> GLPTMLTPGSNQFLTSDDFQSPSAMPQFDVTPEMKIPGEVHNLMEIAEVDSVVPVNNTKENINSMEAYR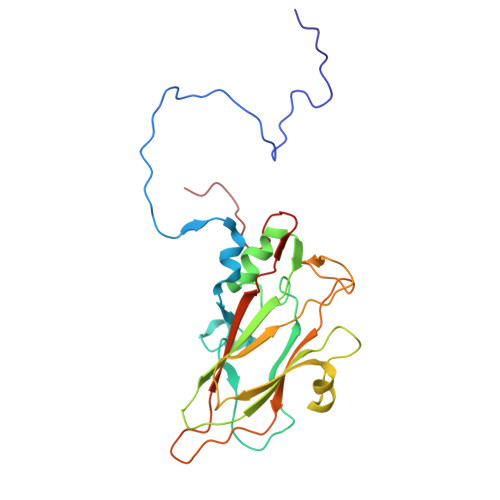IPVTGGDQLHTQVFGFQMQPGLNSVFKRTLLGEILNYYAHWSGSVKLTFVFCGSAMATGKFLLAYSPPGASPPQNRKQAMLGTHVIWDVGLQSSCVLCIPWISQTHYRLVQQDEYTSAGYVTCWYQTGLIVPPGAPPSCTILCFASACNDFSVRNLRDTPFIEQTQLLQ> MKDKVYKRPVSILVVIYAQDTKRVLMLQRRDDPDFWQSVTGSVEEGETAPQAAMREVKEEVTIDVVAEQLTLIDCQRTVEFEIFSHLRHRYAPGVTRNTESWFCLALPHERQIVFTEHLAYKWLDAPAAAALTKSWSNRQAIEQFVINAA

DHNTPase catalyzes the hydrolysis of 7,8-dihydroneopterin triphosphate, the product of GTP cyclohydrolase, to 7,8-dihydroneopterin monophosphate and pyrophosphate. DHNTPase belongs to the Nudix hydrolase superfamily (InterPro IPR000086; Pfam PF00293), which catalyze the hydrolysis of a variety of phosphorylated nucleotide molecules and their derivatives, as well as some non-nucleotide substrates like DHNTP. The motif RExxEE binds a required metal ion cofactor, presumed physiologically to be Mg2+. To better understand how DHNTPase catalyzes its reaction and drive drug discovery efforts, we solved crystal structures of apo, Co2+-, and Ni2+- bound DHNTPase in a new crystal form.

Optimized crystals grown in ~35% PEG 8000, 0.05 mM ammonium sulfate were soaked in a range of dihydroneopterin concentrations and either 10 mM MgSO4, NiCl2, or 5 mM CoCl2. We solved the respective three ~2 Å resolution structures in space group C2 containing one monomer per asymmetric unit. Although crystals soaked with Mg2+ contained only water molecules in the active site (not shown), those soaked with Co2+ or Ni2 appeared to be metallated. Second, based on the fact that the Mg-soaked crystals contained only water, we infer that metal loading in DHNTPase is substrate-assisted, like other Mg-dependent enzymes involving nucleotide substrates. The main difference between our structures and those previously reported is that there is no shift in loops labeled L2 and L5, which was proposed to be a conformational change needed for catalysis. Notably, in the absence of metal, sulfate binding to apo DHNTPase is detectable, and associated with +1°C thermal stabilization. ITC data could only be fit by a sequential binding model with stoichiometry of n = 2, taking advantage of the a priori knowledge that two sulfates were observed crystallographically in the apo structure, one in the active site and the other on the surface ~ 20 Å away. We suggest that the higher Ka site corresponds to the active site sulfate, and may be a distorted binding site utilizing positively charged Arg29 and/or Lys7 in this region, and the second site is the one stabilized by Trp136 and Arg97 remote from the active site. In silico docking of the substrate DHNTP to apo DHNTPase followed by minor manual adjustment in the metal binding region reveals a binding pose compatible with the metallated structures, its bound sulfate anion, and the previous PPi-bound structures.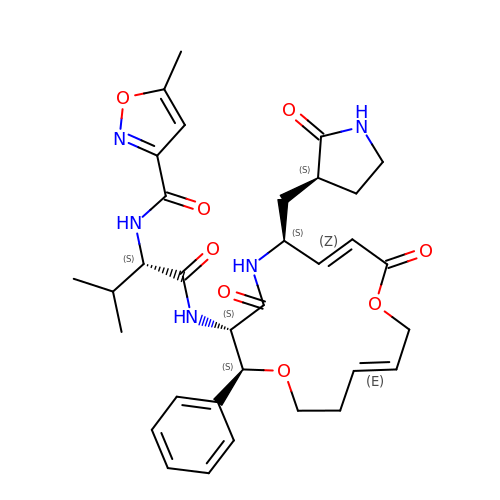~{N}-[(2~{S})-1-[[(2~{S},3~{S},6~{S},7~{Z},12~{E})-4,9-bis(oxidanylidene)-6-[[(3~{S})-2-oxidanylidenepyrrolidin-3-yl]methyl]-2-phenyl-1,10-dioxa-5-azacyclopentadeca-7,12-dien-3-yl]amino]-3-methyl-1-oxidanylidene-butan-2-yl]-5-methyl-1,2-oxazole-3-carboxamide | C33 H41 N5 O8 | XPQNIWALCQRNAP-GPCDZKPZSA-N>GASEPSGPPTDLWVESRGPFTILVRWKAPPKEYWHGKLKGYYVGYKMEGSPQPYSFKTVEAMNVNITHEYLLNSLKKSTKYSIVVKAYNAAGTGPASQELIVKTLDGVLPRPPSVSLLSASDSTISVKWGHT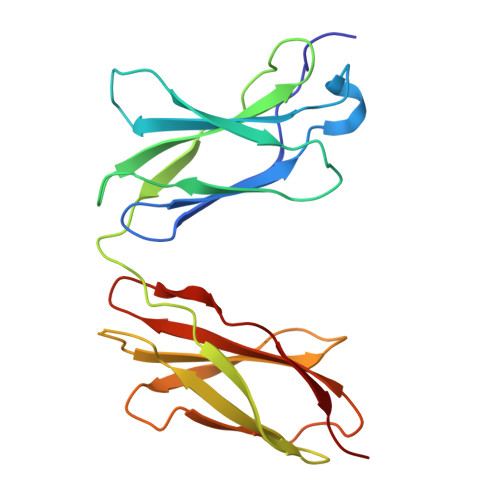ISRDEPVTGYTLHYRKKVGHWLHVPLLASDQTRYTLTGLDSDTTYNVYVTANNRYGRGDPSGILSVRTGD[7x]> GADSPVLMVYGLDQSKMNCDRVFNVFCLYGNVEKVKFMKSKP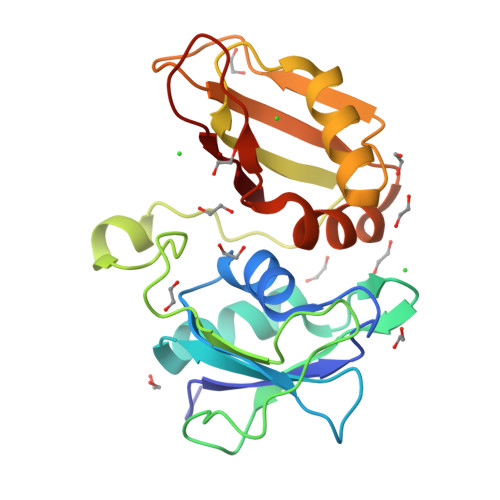GAAMVEMADGYAVDRAITHLNNNFMFGQKMNVCVSKQPAIMPGQSYGLEDGSCSYKDFSESRNNRFSTPEQAAKNRIQHPSNVLHFFNAPLEVTEENFFEICDELGVKRPTSVKVFSGKSERSSSGLLEWDSKSDALETLGFLNHYQMKNPNGPYPYTLKLCF> GHMNITDIREQFPILHQQVNGHDLVYLDSAATSQKPRAVIETLDKYYNQYNSNVHRGVHTLGTRATDGYEGAREKVRKFINAKSMAEIIFTKGTTTSLNMVALSYARANLKPGDEVVITYMEAHANIIPWQQAVKATGATLKYIPLQEDGTISLEDVRETVTSNTKIVAVSHVSNVLGTVNPIKEMAKIAHDNGAVIVVDGAQSTPHMKIDVQDLDCDFFALSSHKMCGPTGVGVLYGKKALLENMEPAEFGGEMIDFVGLYESTWKELPWKFEAGTPIIAGAIGLGAAIDFLEEIGLDEISRHEHKLAAYALERFRQLDGVTVYGPEERAGLV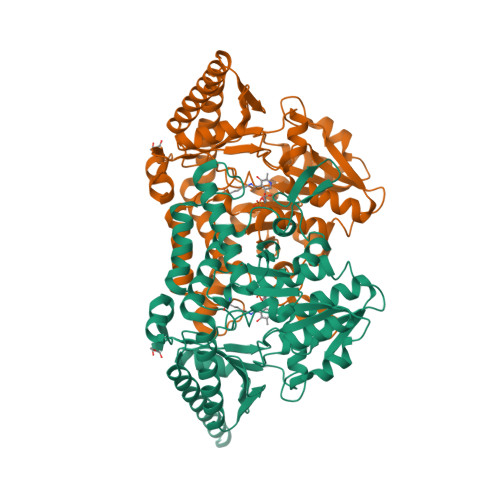TFNLDDVHPHDVATVLDAEGIAVRAGHHCAQPLMKWLDVTATARASFYLYNTEEEIDKLVEALQKTKEYFTNVFVDLEHHHHHH In siphophage T5, the unique RBP is located at the extremity of a central fiber. FhuA, an outer membrane E. coli iron-ferrichrome transporter, is the bacterial receptor recognized by T5 (25). We present the structures of T5 tail tip, determined by cryo–electron microscopy before and after interaction with its E. coli receptor, FhuA, reconstituted into nanodisc. These structures bring out the important conformational changes undergone by T5 tail tip upon infection, which include bending of T5 central fiber on the side of the tail tip, tail anchoring to the membrane, tail tube opening, and formation of a transmembrane channel.

(C) Cryo-EM structure of T5 upper tail tip at 3.5-Å resolution. After two TTPpb6 trimeric rings, the tube continues with a p140 trimer and then a DTPpb9 hexamer. A BHPpb3 trimer closes the tube and forms the beginning of the central fiber that continues with a pb4 trimer. A long linker runs along the protein down to the tip of the cone, inserted between two neighboring BHPpb3 subunits and contributing to the stability of the closed tube. BHPpb3 C terminus forms the beginning of the central fiber with two fibronectin domains (FNIII), further stabilizing the closed tube and giving BHPpb3 the shape of a trophy cup. BHPpb3 results from a tail tube domain duplication/fusion, as TTPpb6. TMPpb2 density is very ill-defined along the tail tube, probably due to a poor interaction network between the predicted coiled-coil of TMPpb2* and the wall of the tube, except in the BHPpb3 cup. There, we could model TMPpb2C 35 C-terminal residues. Three TMPpb2C copies are coiled in a superhelix, burying hydrophobic residues in its center, interacting closely with BHPpb3 plug.

>[6x]MSLQLLRNTRIFVSTVKTGHNKTNTQEILVQDDISWGQDSNSTDITVNEAGPRPTRGSKRFNDSLNAAEWSFSTYILPYKDKNTSKQIVPDYMLWHALSSGRAINLEGTTGAHNNATNFMVNFKDNSYHELAMLHIYILTDKTWSYIDSCQINQAEVNVDIEDIGRVTWSGNGNQLIPLDEQPFDPDQIGIDDETYMTIQGSYIKNKLTILKIKDMDTNKSYDIPITGGTFTINNNITYLTPNVMSRVTIPIGSFTGAFELTGSLTAYLNDKSLGSMELYKDLIKTLKVVNRFEIALVLGGEYDDERPAAILVAKQAHVNIPTIETDDVLGTSVEFKAIPSDLDAGDEGYLGFSSKYTRTTINNLIVNGDGATDAVTAITVKSAGNVTTLNRSATLQMSVEVTPSSARNKEVTWAITAGDAATINATGLLRADASKTGAVTVEATAKDGSGVKGTKVITVTAGG;>[3x]MFYSLMRESKIVIEYDGRGYHFDALSNYDASTSFQEFKTLRRTIHNRTNYADSIINAQDPSSISLAINFSTTLIESNFFDWMGFTREGNSLFLPRNTPNIEPIMFNMYIINHNNSCIYFENCYVSTVDFSLDKSIPILNVGIESGKFSEVSTFRDGYTITQGEVLPYSAPAVYTNSSPLPALISASMSFQQQCSWREDRNIFDINKIYTNKRAYVNEMNASATLAFYYVKRLVGDKFLNLDPETRTPLIIKNKYVSITFPLARISKRLNFSDLYQVEYDVIPTADSDPVEINFFGERK;>[12x]MSTENRVIDLVVDENVPYGLLMQFMDVDDSVYPSTSKPVDLTDFSLRGSIKSSLEDGAETVASFTTAIVDAAQGVASISLPVSAVTTIASKASKERDRYNPRQRLAGYYDVIITRTAVGSAASSFRIMEGKVYISDGVTQ;>[6x]MRLPDPYTNPEYPGLGFESVNLVDNDPMIRDELPNGKVKEVKISAQYWGINISYPELFPDEYAFLDSRLLEYKRTGDYLDVLLPQYEAFRVRGDTKSVTIPAGQKGSQIILNTNGTLTGQPKAGDLFKLSTHPKVYKITNFSSSGNVWNISLYPDLFITTTGSEKPVFNGILFRTKLMNGDSFGSTLNNNGTYSGISLSLRESL;>[3x]MKKILDSAKNYLNTHDKLKTACLIALELPSSSGSAATYIYLTDYFRDVTYNGILYRSGKVKSISSHKQNRQLSIGSLSFTITGTAEDEVLKLVQNGVSFLDRGITIHQAIINEEGNILPVDPDTDGPLLFFRGRITGGGIKDNVNTSGIGTSVITWNCSNQFYDFDRVNGRYTDDASHRGLEVVNGTLQPSNGAKRPEYQEDYGFFHSNKSTTILAKYQVKEERYKLQSKKKLFGLSRSYSLKKYYETVTKEVDLDFNLAAKFIPVVYGVQKIPGIPIFADTELNNPNIVYVVYAFAEGEIDGFLDFYIGDSPMICFDETDSDTRTCFGRKKIVGDTMHRLAAGTSTSQPSVHGQEYKYNDGNGDIRIWTFHGKPDQTAAQVLVDIAKKKGFYLQNQNGNGPEYWDSRYKLLDTAYAIVRFTINENRTEIPEISAEVQGKKVKVYNSDGTIKADKTSLNGIWQLMDYLTSDRYGADITLDQFPLQKVISEAKILDIIDESYQTSWQPYWRYVGWNDPLSENRQIVQLNTILDTSESVFKNVQGILESFGGAINNLSGEYRITVEKYSTNPLRINFLDTYGDLDLSDTTGRNKFNSVQASLVDPALSWKTNSITFYNSKFKEQDKGLDKKLQLSFANITNYYTARSYADRELKKSRYSRTLSFSVPYKFIGIEPNDPIAFTYERYGWKDKFFLVDEVENTRDGKINLVLQEYGEDVFINSEQVDNSGNDIPDISNNVLPPRDFKYTPTPGGVVGAIGKNGELSWLPSLTNNVVYYSIAHSGHVNPYIVQQLENNPNERMIQEIIGEPAGLAIFELRAVDINGRRSSPVTLSVDLNSAKNLSVVSNFRVVNTASGDVTEFVGPDVKLAWDKIPEEEIIPEIYYTLEIYDSQDRMLRSVRIEDVYTYDYLLTYNKADFALLNSGALGINRKLRFRIRAEGENGEQSVGWATI;>[3x]MTDKLIRELLIDVKQKGATRTAKSIENVSDALENAAAASELTNEQLGKMPRTLYSIERAADRAAKSLTKMQASRGMAGITKSIDGIGDKLDYLAIQLIEVTDKLEIGFDGVSRSVKAMGNDVAAATEKVQDRLYDTNRALGGTSKGFNDTAGAAGRASRALGNTSGSARGATRDFAAMAKIGGRLPIMYAALASNVFVLQTAFESLKVGDQLNRLEQFGTIVGTMTGTPVQTLALSLQNATNGAISFEEAMRQASSASAYGFDSEQLEQFGLVARRAAAVLGVDMTDALNRVIKGVSKQEIELLDELGVTIRLNDAYENYVKQLNATSTGIKYTVDSLTTYQKQQAYANEVIAESTRRFGYLDDALKATSWEQFAANANSALRSLQQSAATYLNPVMDTLNTFLYQTKSSQMRVSAMARSASAKTTPAENVTALIENAVGAREDLDTYLKESEERVKKAQELKQQLDDLKAKQAATAPIANALTAGGIGGDESNKLVVQLTNELARQNKEIEERTKTEKVLRQAVQDTGEALLRNGKLAEQLGAKMKYADTAVPGDKGVFEVDPNNLKAVSEIQKNFDFLKKSSSDTANNIRMAASSITNAKKASSDLNSVVKAVEDTSKVTGQSADTLVKNLNLGFSSLDQMKAAQKGLSEYVTAMDKSEQNALEVAKRKDEVYNQTKDKAKAEAAAREVLLRQQQEQLTAAKALLAINPNDPEALKQVAKIETEILNTKAQGFENAKKTKDYTDKILGVDREIALLNDRTMTSTQYRLAQLRLELQLEQEKTELYSKQADGQAKVEQSRRAQAQISREIWEAEKQGTASHVSALMDALEVSQTQRNVTGQSQILTERLSILQQQLELSKGNTEEELKYRNEIYKTSAALEQLKKQRESQMQQQVGSSVGATYTSTTGLIGEDKDFADMQNRMASYDQAISKLSELNSEATAVAQSMGNLTNAMIQFSQGSLDTTSMIASGMQTVASMIQYSTSQQVSAIDQAIAAEQKRDGKSEASKAKLKKLEAEKLKIQQDAAKKQIIIQTAVAVMQAATAVPYPFSIPLMVAAGLAGALALAQASSASGMSSIADSGADTTQYLTLGERQKNVDVSMQASSGELSYLRGDKGIGNANSFVPRAEGGMMYPGVSYQMGEHGTEVVTPMVPMKATPNDQLSDGSKTTSGRPIILNISTMDAASFRDFASNNSTAFRDAVELALNENGTTLKSLGNS>[2x]GSAKDPMTELKQADQIRTWVQSVLTGESSGHDWLHISRVADLAVYIGEKENADLFIVETAALVHDLIDVKLPDTIRLSVSEVYNQLVTFGIGKEDAD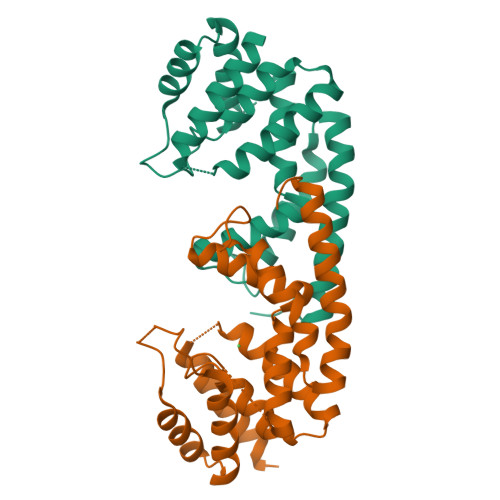RVIHIITKMSFRDREKLEGEPLSIEGKVVQDADRLDAIGAVGIARAFMFAGAKGHGLYGDDQSAYAHFFHKLLRLIDMMNTDTARELAEERHEFMLQYIRQLEKDIPGIDAKTS> MGALLDRFSGDEKKGRLIEAVCGQDLVANDKDLAEQIVAAGVLQEIADGDVIIKQGDWDDDLFLILAGKMQITINGRPQTVREAGTHVGELTGTSPARPRTATVSAIGEALVLRLKRTVLDEITRDSPAYLKRMLDVVAGRLDERNKGIGQTNDIPRIFVISSSEKIGVANEIVRNLDSKEIAVQLWDKGTFGISDYPISSLMDAIESSDFTIAVVGADDTLTMRGETHQVARDNVHLEFGISLG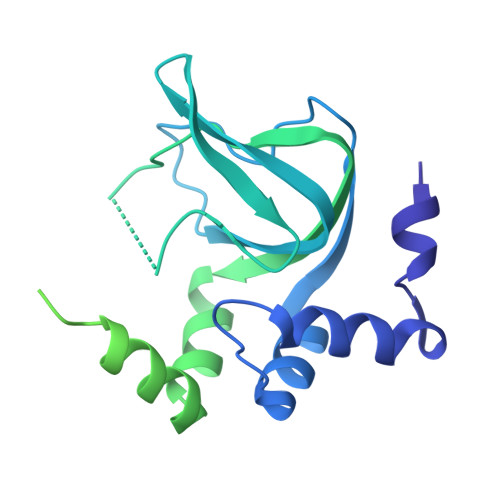VLGRRRSMLLVCADDGVRLPSDAAGLTTLRYRTGSDDEMKRTVRNACIEAKEHIEKEGVFTDRRAR> MMSDQENENEHAKAFLGLAKCEEEVDAIEREVELYRLNKMKPVYEKRDAYI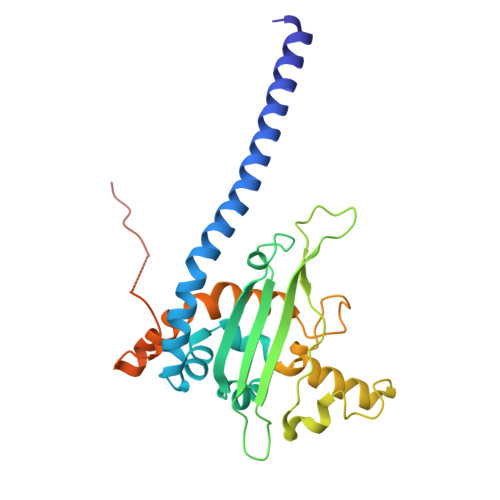DEIAEFWKIVLSQHVSFANYIRASDFKYIDTIDKIKVEWLALESEMYDTRDFSITFHFHGIEGDFKEQQVTKVFQIKKGKDDQEDGILTSEPVPIEWPQSYDSINPDLIKDKRSPEGKKKYRQGMKTIFGWFRWTGLKPGKEFPHGDSLASLFSEEIYPFCVKYYAEAQRDLEDEEGESGLSADGDSEDDDGSLGEVDLPLSDEEPSSKKRKV> AAIDPNRIVALEWLPVELLLALGIVPYGVADTINYRLWVSEPPLPDSVIDVGLRTEPNLELLTEMKPSFMVWSAGYGPSPEMLARIAPGRGFNFSDGKQPLAMARKSLTEMADLLNLQSAAETHLAQYEDFIRSMKPRFVKRGARPLLLTTLIDPRHMLVFGPNSLFQEILDEYGIPNAWQGETNFWGSTAVSIDRLAAYKDVDVLCFDHDNSKDMDALMATPLWQAMPFVRA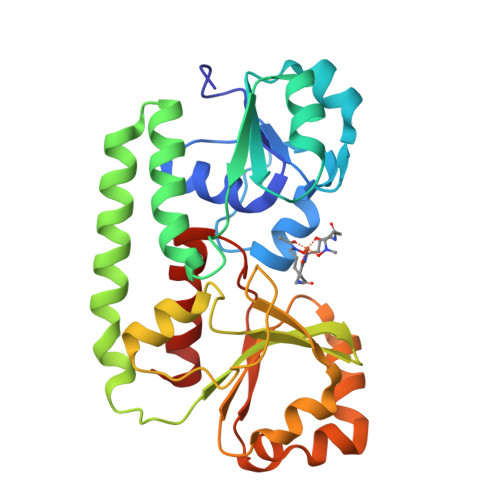GRFQRVPAVWFYGATLSAMHFVRVLDNAIGGKA>MSQRITIDPVTRIEGHLRIDCEIENGVVSKAWASGTMWRGMEEIVKNRDPRDAWMIVQRICGVCTTTHAISSVRAAESALNIDVPVNAQYIRNIILAAHTTHDHIVHFYQLSALDWVDITSALKADPAKASAMLNGVSTWHLNSAEEFTKVQNKIKDLVASGQLGIFANGCWGHPAMQLPPEVNLIAVAHYLQALECQRDANRVVALLGGKTPHIQNLAVGGVANPINLDGLGVLNLERLMYIKSFIDKLSDFVEQVYKVDTAVIAAFYPEWLERGQGAVNYLSAPEFPTDGKNGSFLFPGGYITDADLSTYRPITSHSDEYLIKGIQESAKHAWYKDEAPQAPWEGTTVPDYTGWSDDGKYSWVKAPTFYGKTVEVGPLANMLCKLAAKRESTHAKLNEIVAIYTKLTGKTIEVAQLHSTLGRIIGRTVHCCELQNVLQDQYNALIVNIGKGDHTTFVKPDIPATGEFKGVGFLEAPRGMLSHWMVIKDGIISNYQAVVPSTWNSGPRNFNDEVGPYERSLVGTPIADPNKPLEVVRTIHSFDPCMSCAVH[2x];>[2x]EMAESVSRPQRPP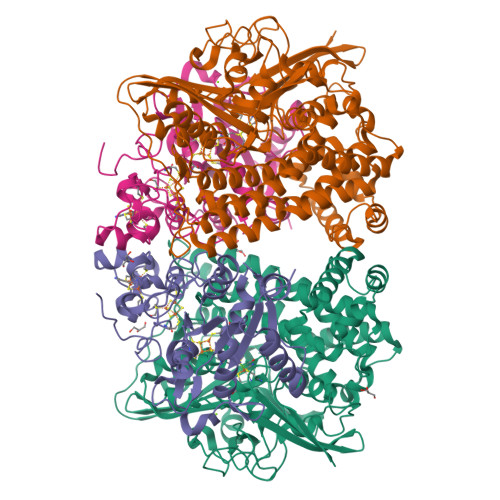VIWIGAQECTGCTESLLRATHPTVENLVLETISLEYHEVLSAAFGHQVEENKHNALEKYKGQYVLVVDGSIPLKDNGIYCMVAGEPIVDHIRRAAEGAAAIIAIGSCAAWGGVAAAGVNPTGAVGLQEVLPGKTIINIPGCPPNPHNFLATVAHIITYGKPPKLDAKNRPTFAYGRLIHEHCERRPHFDAGRFAKEFGDEGHREGWCLYHLGCKGPETYGNCSTLQFCDVGGVWPVAIGHPCYGCNEEGIGFHKGIHQLAHVENQTPRSEKPDVNIKEGGNISAGAVGLLGGVVGLVAGVSVMAVRELGRQQKKDNADSRGE N-[4-({3-[2-(methylamino)pyrimidin-4-yl]pyridin-2-yl}oxy)naphthalen-1-yl]-6-(trifluoromethyl)-1H-benzimidazol-2-amine | C28 H20 F3 N7 O | 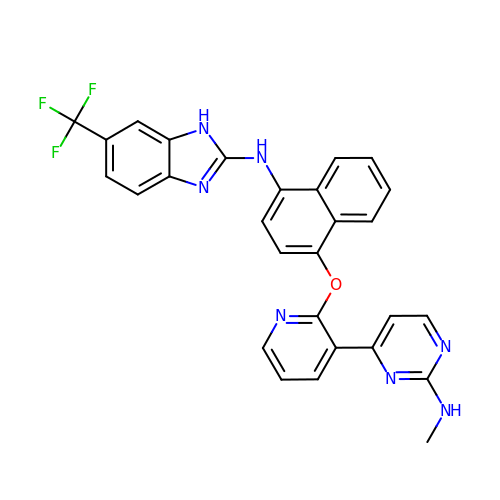VIHXUAKPZPXVSW-UHFFFAOYSA-N> EDLLKNLLTMGVDIDMARKRQPGVFHRMITNEQDLKMFLLSKGASKEVIASIISRYPRAITRTPENLSKRWDLWRKIVTSDLEIVNILERSPESFFRSNNNLNLENNIKFLYSVGLTRKCLCRLLTNAPRTFSNSLDLNKQMVEFLQAAGLSLGHNDPADFVRKIIFKNPFILIQSTKRVKANIEFLRSTFNLNSEELLVLICGPGAEILDLS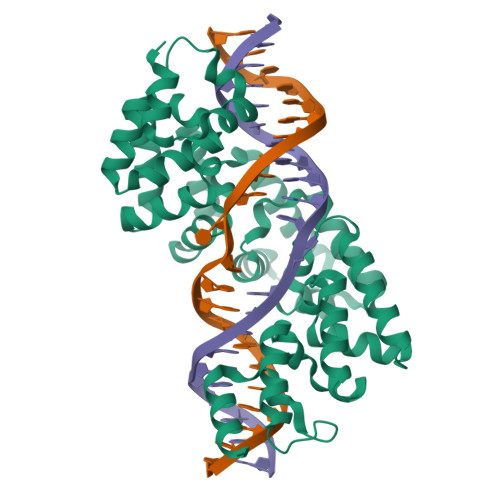NDYARRSYANIKEKLFSLGCTEEEVQKFVLSYPDVIALAEKKFNDKIDCLMEENISISQIIENPRVLDSSISTLKSRIKELVNAGCNLSTLNITLLSWSKKRYEAKLKKLS> SEFVATTGDITVSVSTSFLPELSSVHP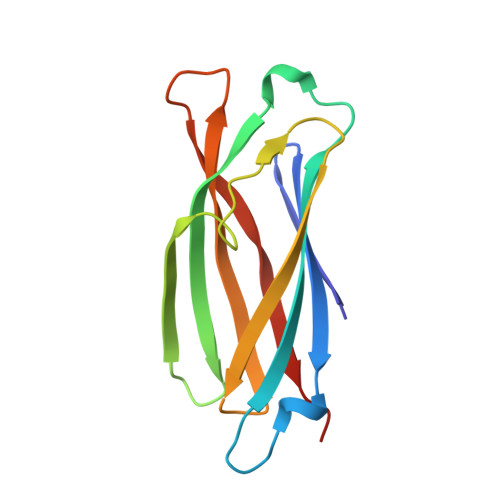PHYFFTYRIRIEMSKDALPEKACQLDSRYWRITNAKGDVEEVQGPGVVGEFPIISPGRVYEYTSCTTFSTTSGYMEGYYTFHFLYFKDKIFNVAIPRFHMACPTFR> KETAAAKFERQHMDSSTSAASSSNYCNQMMKSRNLTKDRCK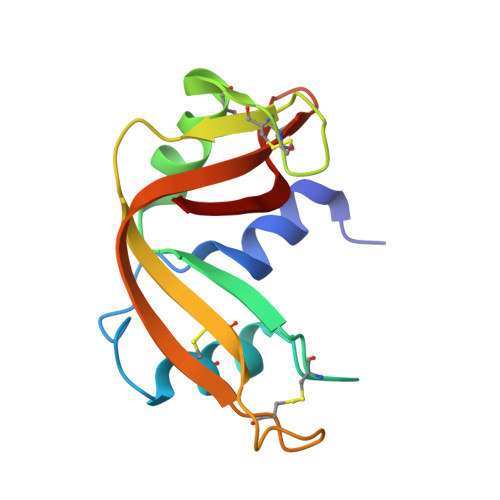PVNTAVHESLADVQAVCSQKNVACKNGQTNCYQSYSTMSITDCRETGSSKYPNCAYKTTQANKHIIVACEGNPYVPVHFDASV(3R)-3-{3-[(1-benzofuran-3-yl)methyl]-1,2,4-oxadiazol-5-yl}-4-cyclopentyl-N-hydroxybutanamide | C20 H23 N3 O4 | 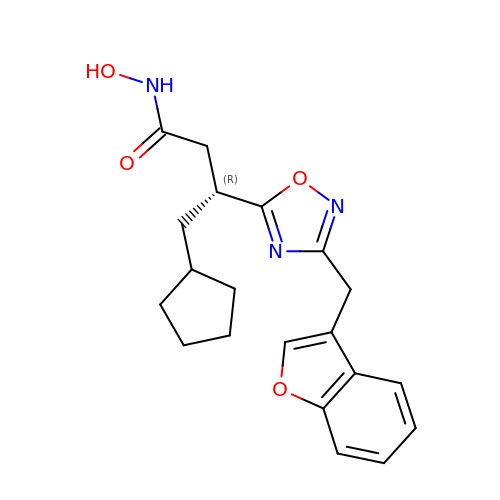CCFPWVUEYLWVCR-CQSZACIVSA-N> MHHHHHHSSGMNVPVGHLRNVQVLGIDAGGTMTDTFFVDQDGDFVVGKAQSTPQNEALGLIASSEDGLANWGMSLHEALAQLQTGVYSGTAMLNRVVQRKGLKCGLIVNRGMEDFHRMGRAVQSHLGYAYEDRIHLNTHRYDPPLVPRHLTRGVVERTDMIGTQVIPLREDTARDAARDLIAADAEGIVISLLHSYKNPENERRVRDIVLEEVEKSGKKIPVFASADYYPVRKETHRTNTTILEGYAAEPSRQTLSKISNAFKERGTKFDFRVMATHGGTISWKAKELARTIVSGPIGGVIGAKYLGEVLGYKNIACSDIGGTSFDVALITQGEMTIKNDPDMARLVLSLPLVAMDSVGAGAGSFIRLDPYTRAIKLGPDSAGYRVGVCWKESGIETVTISDCHMVLGY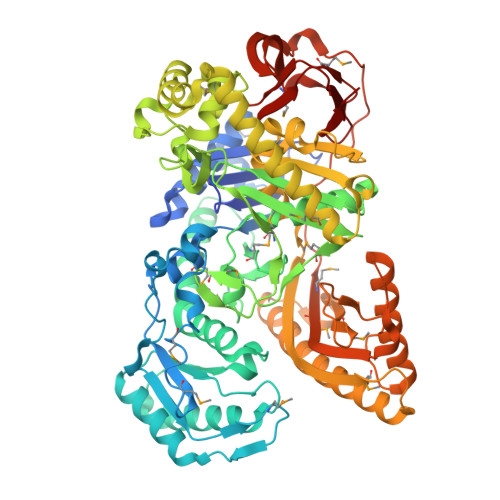LNPDNFLGGAVKLDRQRSVDAIKAQIADPLGLSVEDAAAGVIELLDSDLRDYLRSMISGKGYSPASFVCFSYGGAGPVHTYGYTEGLGFEDVIVPAWAAGFSAFGCAAADFEYRYDKSLDINMPTETPDTDKEKAAATLQAAWEELTKNVLEEFKLNGYSADQVTLQPGYRMQYRGQLNDLEIESPLAQAHTAADWDQLTDAFNATYGRVYAASARSPELGYSVTGAIMRGMVPIPKPKIPKEPEEGETPPESAKIGTRKFYRKKRWVDAQLYHMESLRPGNRVMGPAVIESDATTFVVPDGFETWLDGHRLFHLREV>[4x]SQTLRIGYVSSLLYGLLPEIIYLFRQQNPEIHIELIECGTKDQINALKQGKIDLGFGRLKITDPAIRHIVLHKEQLKLAIHKHHHLNQFAATGVHLSQI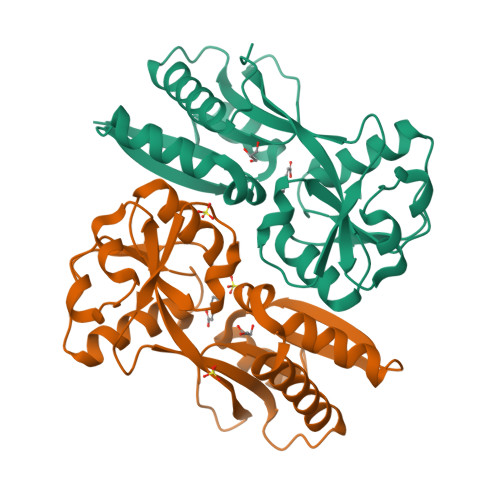IDEPMLLYPVSQKPNFATFIQSLFTELGLVPSKLTEIREIQLALGLVAAGEGVCIVPASAMDIGVKNLLYIPILDDDAYSPISLAVRNMDHSNYIPKILACVQEVFATHHIRPLIESILEHHHHHH The small-molecule compound erastin induces ferroptosis via inhibiting the cystine-glutamate antiporter system xc–, which consists of two subunits, namely the light chain xCT and the heavy chain 4F2hc (encoded by the SLC7A11 and SLC3A2 genes, respectively). The complex formed by xCT and 4F2hc has also been suggested as a possible therapeutic target for cancer, as it is overexpressed in a wide variety of cancer types; moreover, inhibiting xCT impairs cystine uptake, causing an accumulation of ROS and suppressing tumor growth. Erastin functions by inhibiting the import of cystine, thereby depleting intracellular glutathione (GSH), which serves as a necessary cofactor for the enzyme glutathione peroxidase 4 (GPX4) in eliminating lipid peroxides.

Here, we used cryogenic electron microscopy (cryo-EM) to determine the structure of the erastin-bound xCT–4F2hc complex at 3.4 Å resolution. Using this approach, nearly all of the sequences in both the xCT and 4F2hc subunits were resolved, with the exceptions of N-terminal residues 1–45 in xCT and N-terminal residues 1–163 in 4F2hc, which were not visible in the cryo-EM map. The overall structure of the xCT–4F2hc complex is similar to that of the previously reported complex between the l-type amino acid transporter 1 (LAT1) and 4F2hc11, with xCT in an inward-facing conformation. 4F2hc interacts with xCT at the extracellular interface and in the transmembrane region mainly through polar and hydrophobic interactions, respectively. The Cys158 residue in xCT forms a disulfide bond with the Cys211 residue in 4F2hc, and two lipid molecules bind to xCT at the transmembrane region near the intracellular side. Finally, the residues in 4F2hc that precede the transmembrane (TM) helix form a short helix (H1′) that fixes xCT at the intracellular side. We also observed a well-resolved non-protein density in the intracellular vestibule of xCT, into which we incorporated an erastin molecule in the model, as the shape of this density is consistent with erastin. This erastin molecule fit well into the intracellular vestibule and was sandwiched between the TM domains of the xCT subunit. In this complex, the chlorophenoxy group in the erastin molecule functionally interacts with the Phe254 residue in the TM6b domain of xCT, thereby mediating erastin’s inhibitory effects of erastin and regulating erastin-induced ferroptosis; consistent with the finding that the chlorophenoxy moiety is required for inducting ferroptosis. We found that cells expressing the F254A mutant were less sensitive to erastin-induced inhibition of cystine uptake.

> MAHHHHHHHHHHSGRELQPPEASIAVVSIPRQLPGSHSEAGVQGLSAGDDSETGSDCVTQAGLQLLASSDPPALASKNAEVTVETGFHHVSQADIEFLTSIDPTASASGSAGITGTMSQDTEVDMKEVELNELEPEKQPMNAASGAAMSLAGAEKNGLVKIKVAEDEAEAAAAAKFTGLSKEELLKVAGSPGWVRTRWALLLLFWLGWLGMLAGAVVIIVRAPRCRELPAQKWWHTGALYRIGDLQAFQGHGAGNLAGLKGRLDYLSSLKVKGLVLGPIHKNQKDDVAQTDLLQIDPNFGSKEDFDSLLQSAKKKSIRVILDLTPNYRGENSWFSTQVDTVATKVKDALEFWLQAGVDGFQVRDIENLKDASSFLAEWQNITKGFSEDRLLIAGTNSSDLQQILSLLESNKDLLLTSSYLSDSGSTGEHTKSLVTQYLNATGNRWCSWSLSQARLLTSFLPAQLLRLYQLMLFTLPGTPVFSYGDEIGLDAAALPGQPMEAPVMLWDESSFPDIPGAVSANMTVKGQSEDPGSLLSLFRRLSDQRSKERSLLHGDFHAFSAGPGLFSYIRHWDQNERFLVVLNFGDVGLSAGLQASDLPASASLPAKADLLLSTQPGREEGSPLELERLKLEPHEGLLLRFPYAALE;> MADYKDDDDKSGPDEVDASGRVRKPVVSTISKGGYLQGNVNGRLPSLGNKEPPGQEKVQLKRKVTLLRGVSIIIGTIIGAGIFISPKGVLQNTGSVGMSLTIWTVCGVLSLFGALSYAELGTTIKKSGGHYTYILEVFGPLPAFVRVWVELLIIRPAATAVISLAFGRYILEPFFIQCEIPELAIKLITAVGITVVMVLNSMSVSWSARIQIFLTFCKLTAILIIIVPGVMQLIKGQTQNFKDAFSGRDSSITRLPLAFYYGMYAYAGWFYLNFVTEEVENPEKTIPLAICISMAIVTIGYVLTNVAYFTTINAEELLLSNAVAVTFSERLLGNFSLAVPIFVALSCFGSMNGGVFAVSRLFYVASREGHLPEILSMIHVRKHTPLPAVIVLHPLTMIMLFSGDLDSLLNFLSFARWLFIGLAVAGLIYLRYKCPDMHRPFKVPLFIPALFSFTCLFMVALSLYSDPFSTGIGFVITLTGVPAYYLFIIWDKKPRWFRIMSEKITRTLQIILEVVPEEDKL>MVKVDLESKRYGEKLKEVFLMLDNNVVECIKEITESSRNGKLVFFVGAGVSTLSDYPQWWRLVDKYHEELYGSPKKGNYSSDEYLRIPQIFYNVKGEMAFDGILKDFFQVDKPTNPIHDKILAMNPAHVITTNYDNLIDTACWKRGKYFSVISAEEDVANATSSRYLLKVHGDFRKGFKGENVVLKEDDYLNYDQNYPLISNLMKTIIATHTIVFIGYGLGDYNINMLLNWVRKLQKDSFHKPFFIRTDPSPIENETLIYYENKGLRIIDAASLIDSNEYDYLERYSAVMDLLIESQENKFITKDDEVIDYIYGKISPLFALQYIRKIDLKHVFEYDYHFEVNGTVVRHKNKGFGYMERFFELKESCDERSKLSKKQYERFNALFNFFEKNGVICMAKDAGTLNTSIEINSLAYHGKYDVMKKFIEEQSVSIEDDYKKAFFLACLGRWEESYDLYSNIILNSIDESNGCVYYLSQINRYRIYQSITQAVTQFNGLGLLTFGRHYKPFTDEFLARIERE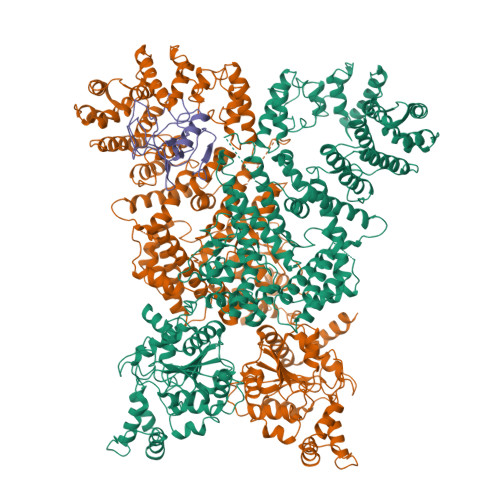MTNFNIDDLFNGMPFEFQKKYKILEFLSDNQFLYDDTVKLFELTNKVRSEMSEGSYSFGMSSDIVVLLRLYDNLRFLYENCLWSVSFHEFHQYIRNSMSLLIEKAEYERTRDIDELGFSFFGKKSGFFMEYYDFVNISRHFKIDDIKNLERSCSIDKIRFGEQEKIEEYLVGIAEEITKQFSANGMNVVFYTQFISEAKAALYFAKYVKLSEEGLGKIVKALLFYFPERDLDIGKRYVWLERLTKCNELPKSIISIIDDFLVLQAEKHIDQNYSEVSSNGLYSRDYGALIKHFEKNFISKRLSEITLCLTQDKQKQIDFLFKLLPLLSTNAKSHLLSFKSVENINDLMNGIRIGLIDEFTPEHEELIIEYLETRKVNYIVEKEKGIQTFSSNDYMSTFGIWYFLEEINNSKMEEFIGMDDQYDFFVDPENFDYKKFIPSWLKNYNDKLLGKIAGNKHMKHHVIEVLKERVKNSNDKRYLEILMNYFI[2x];> MIEIFKDTGATHDLVYHSKINTFVWDVEFDIVLSDSKELNKCYFVKCFNPYRINGKCDFAVSSIDIFSEGKRLLIENEFNFKITKAVHVATSKDVTEIVLHLSERISSPFPIVKEVVYLD> GPGSEFELRRQACGRLAVWLSMIGLAQYYKVLVDNGYENIDFITDITWEDLQEIGITKLGHQKKLMLAVRKLAELQKAEYSKYPSGSGSGENLYFQSGSGSGSPEYPLFVTVGDWLDS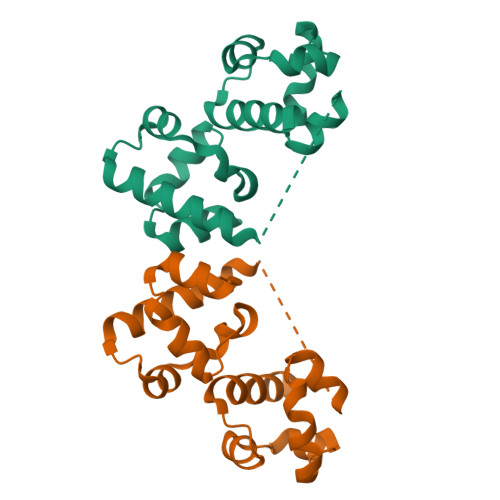IKMGQYKSNFMAAGFTTFDLISRMSIDDIRRIGVILIGHQRRIVSSIQTLRLHMMHIQEKGFHV> MGSDKIHHHHHHENLYFQGMRDHVEIGIGREARRTYSLDDISVVSSRRTRSSKDVDTTWHIDAYKFDLPFMNHPSDALASPEFVIEMGKQGGLGVINAEGLWGRHADLDEAIAKVIAAYEEGDQAAAT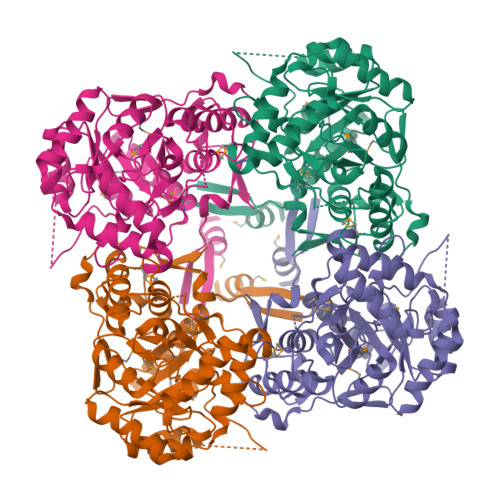RTLQELHAAPLDTELLSERIAQVRDSGEIVAVRVSPQNVREIAPIVIKAGADLLVIQGTLISAEHVNTGGEALNLKEFIGSLDVPVIAGGVNDYTTALHMMRTGAVGIIVGGGENTNSLALGMEVSMATAIADVAAARRDYLDETGGRYVHIIADGSIENSGDVVKAIACGADAVVLGSPLARAEEAAGKGYFWPAVAAHPRFPRGVVTESVDLDEAAPSLEQILHGPSTMPWGVENFEGGLKRALAKCGYTDLKSFQKVSLHVN> MSFPEGKDILFMGNEAAKLAEAFQKSLRKPGHKRSQSIIGKHH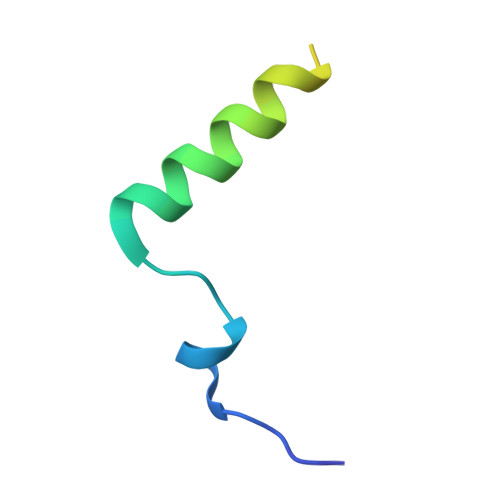HHHH>[2x]MDEAYYSGNLESVLGYVSDMHTELASISQLVIAKIETIDNDILNKDIVNFIMCRSNLDNPFISFLDTVYTIIDQENYQTELINSLDDNEIIDCIVNKFMSFYKDNLENIVDA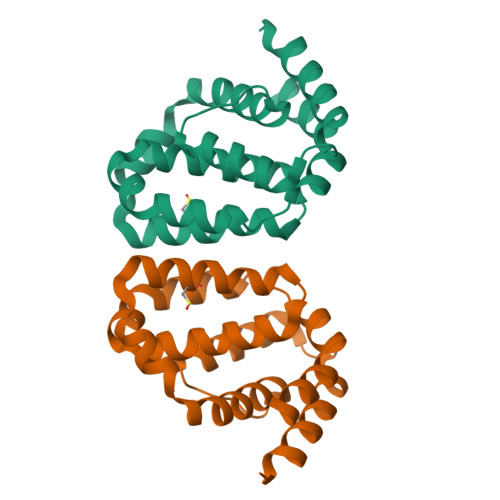IITLKYIMNNPDFKTTYAEVLGSRIADIDIKQVIRENILQLSNDIRERYLKHHHHHH>[4x]MNFSLEGRNIVVMGVANKRSIAWGIARSLHEAGARLIFTYAGERLEKSVHELAGTLDRNDSIILPCDVTNDAEIET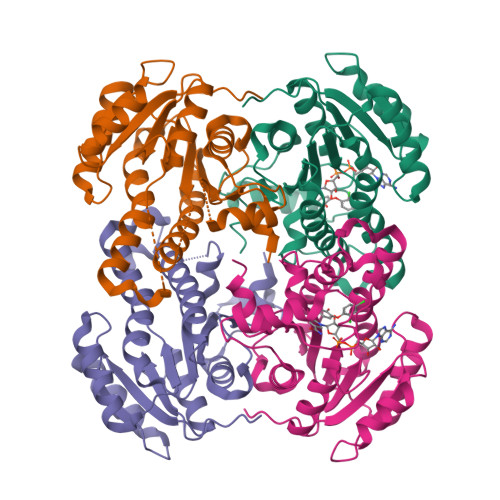CFASIKEQVGVIHGIAHCIAFANKEELVGEYLNTNRDGFLLAHNISSYSLTAVVKAARPMMTEGGSIVTLTYLGGELVMPNYNVMGVAKASLDASVKYLAADLGKENIRVNSISAGPIRTLSAKGISDFNSILKDIEERAPLRRTTTPEEVGDTAAFLFSDMSRGITGENLHVDSGFHITARLEHHHHHH> MDPIINGNSANVYLTDSYLKGVISFSECNALGSYIFNGPYLKNDYTNLISRQNPLIEHMNLKKLNITQSLISKYHKGEIKLEEPTYFQSLLMTYKSMTSSEQIATTNLLKKIIRRAIEISDVKVYAILNKLGLKEKDKIKSNNGQDEDNSVITTIIKDDILSAVKDNQSHLKADKNHSTKQKDTIKTTLLKKLMCSMQHPPSWLIHWFNLYTKLNNILTQYRSNEVKNHGFTLIDNQTLSGFQFILNQYGCIVYHKELKRITVTTYNQFLTWKDISLSRLNVCLITWISNCLNTLNKSLGLRCGFNNVILTQLFLYGDCILKLFHNEGFYIIKEVEGFIMSLILNITEEDQFRKRFYNSMLNNITDAANKAQKNLLSRVCHTLLDKTVSDNIINGRWIILLSKFLKLIKLAGDNNLNNLSELYFLFRIFGHPMVDERQAMDAVKINCNETKFYLLSSLSMLRGAFIYRIIKGFVNNYNRWPTLRNAIVLPLRWLTYYKLNTYPSLLELTERDLIVLSGLRFYREFRLPKKVDLEMIINDKAISPPKNLIWTSFPRNYMPSHIQNYIEHEKLKFSESDKSRRVLEYYLRDNKFNECDLYNCVVNQSYLNNPNHVVSLTGKERELSVGRMFAMQPGMFRQVQILAEKMIAENILQFFPESLTRYGDLELQKILELKAGISNKSNRYNDNYNNYISKCSIITDLSKFNQAFRYETSCICSDVLDELHGVQSLFSWLHLTIPHVTIICTYRHAPPYIGDHIVDLNNVDEQSGLYRYHMGGIEGWCQKLWTIEAISLLDLISLKGKFSITALINGDNQSIDISKPIRLMEGQTHAQADYLLALNSLKLLYKEYAGIGHKLKGTETYISRDMQFMSKTIQHNGVYYPASIKKVLRVGPWINTILDDFKVSLESIGSLTQELEYRGESLLCSLIFRNVWLYNQIALQLKNHALCNNKLYLDILKVLKHLKTFFNLDNIDTALTLYMNLPMLFGGGDPNLLYRSFYRRTPDFLTEAIVHSVFILSYYTNHDLKDKLQDLSDDRLNKFLTCIITFDKNPNAEFVTLMRDPQALGSERQAKITSEINRLAVTEVLSTAPNKIFSKSAQHYTTTEIDLNDIMQNIEPTYPHGLRVVYESLPFYKAEKIVNLISGTKSITNILEKTSAIDLTDIDRATEMMRKNITLLIRILPLDCNRDKREILSMENLSITELSKYVRERSWSLSNIVGVTSPSIMYTMDIKYTTSTISSGIIIEKYNVNSLTRGERGPTKPWVGSSTQEKKTMPVYNRQVLTKKQRDQIDLLAKLDWVYASIDNKDEFMEELSIGTLGLTYEKAKKLFPQYLSVNYLHRLTVSSRPCEFPASIPAYRTTNYHFDTSPINRILTEKYGDEDIDIVFQNCISFGLSLMSVVEQFTNVCPNRIILIPKLNEIHLMKPPIFTGDVDIHKLKQVIQKQHMFLPDKISLTQYVELFLSNKTLKSGSHVNSNLILAHKISDYFHNTYILSTNLAGHWILIIQLMKDSKGIFEKDWGEGYITDHMFINLKVFFNAYKTYLLCFHKGYGKAKLECDMNTSDLLCVLELIDSSYWKSMSKVFLEQKVIKYILSQDASLHRVKGCHSFKLWFLKRLNVAEFTVCPWVVNIDYHPTHMKAILTYIDLVRMGLINIDRIHIKNKHKFNDEFYTSNLFYINYNFSDNTHLLTKHIRIANSELENNYNKLYHPTPETLENILANPIKSNDKKTLNDYCIGKNVDSIMLPLLSNKKLIKSSAMIRTNYSKQDLYNLFPMVVIDRIIDHSGNTAKSNQLYTTTSHQISLVHNSTSLYCMLPWHHINRFNFVFSSTGCKISIEYILKDLKIKDPNCIAFIGEGAGNLLLRTVVELHPDIRYIYRSLKDCNDHSLPIEFLRLYNGHINIDYGENLTIPATDATNNIHWSYLHIKFAEPISLFVCDAELSVTVNWSKIIIEWSKHVRKCKYCSSVNKCMLIVKYHAQDDIDFKLDNITILKTYVCLGSKLKGSEVYLVLTIGPANIFPVFNVVQNAKLILSRTKNFIMPKKADKESIDANIKSLIPFLCYPITKKGINTALSKLKSVVSGDILSYSIAGRNEVFSNKLINHKHMNILKWFNHVLNFRSTELNYNHLYMVESTYPYLSELLNSLTTNELKKLIKITGSLLYNFHNE;>MEKFAPEFHGEDANNRATKFLESIKGKFTSPKDPKKKDSIISVNSIDIEVTKESPITSNSTIINPTNETDDTAGNKPNYQRKPLVSFKEDPTPSDNPF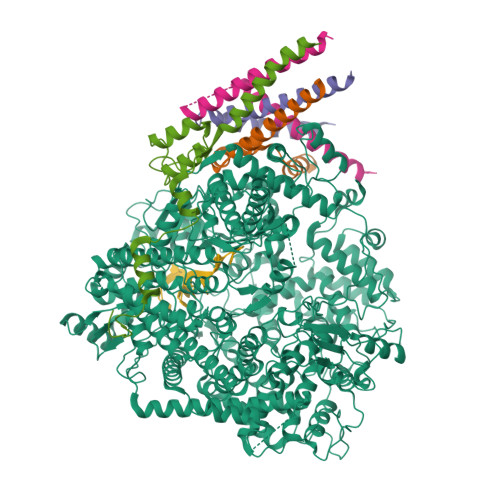SKLYKETIETFDNNEEESSYSYEEINDQTNDNITARLDRIDEKLSEILGMLHTLVVASAGPTSARDGIRDAMVGLREEMIEKIRTEALMTNDRLEAMARLRNEESEKMAKDTSDEVSLNPTSEKLNNLLEGNDSDNDLSLEDF[4x]{4-[3-(4-fluorophenyl)-1H-pyrazol-4-yl]pyridin-2-yl}methanol | C15 H12 F N3 O 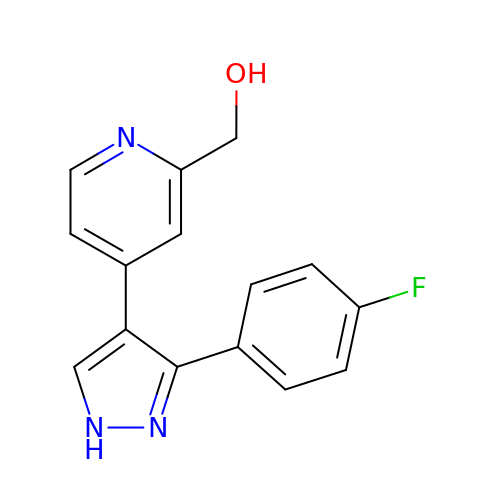| RKBVIYAYFDBXIL-UHFFFAOYSA-N>METPLEKALTTMVTTFHKYSGREGSKLTLSRKELKELIKKELCLGEMKESSIDDLMKSLDKNSDQEIDFKEYSVFLTMLCMAYNDFFLEDNK[2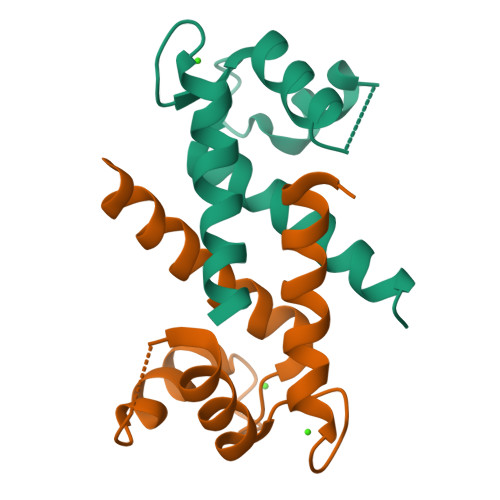x]> IVGGTSASAGDFPFIVSISRNGGPWCGGSLLNANTVLTAAHCVSGYAQSGFQIRAGSLSRTSGGITSSLSSVRVH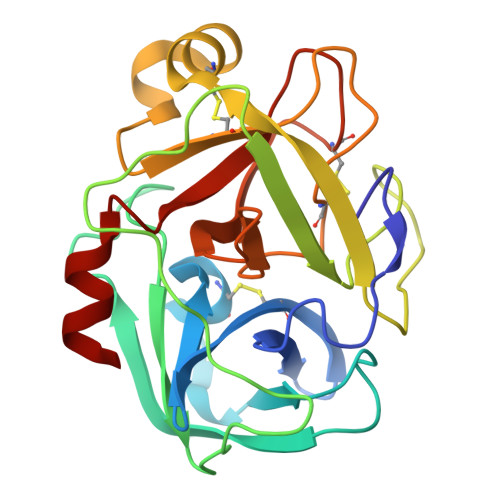PSYSGNNNDLAILKLSTSIPSGGNIGYARLAASGSDPVAGSSATVAGWGATSEGGSSTPVNLLKVTVPIVSRATCRAQYGTSAITNQMFCAGVSSGGKDSCQGDSGGPIVDSSNTLIGAVSWGNGCARPNYSGVYASVGALRSFIDTYA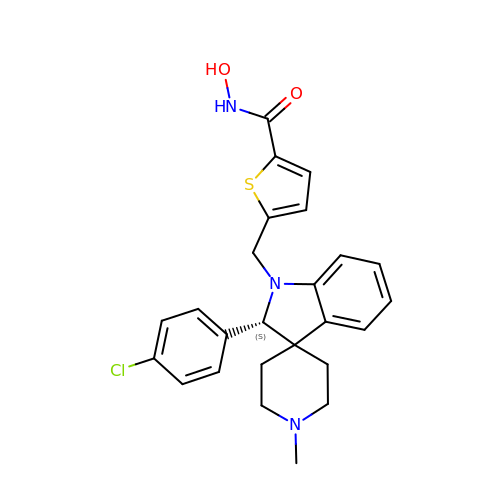5-[[(2S)-2-(4-chlorophenyl)-1'-methyl-spiro[2H-indole-3,4'-piperidine]-1-yl]methyl]-N-oxidanyl-thiophene-2-carboxamide | C25 H26 Cl N3 O2 S | DLQYRYFSBDRUBH-QHCPKHFHSA-N>[2x]GQDLALSCGTSEASADQDKKKWEPDTKFLKTGNSIHATATYQDPSLLSTVPYMTARIFTAPATYEIPIKGDKRHLLRLYFYPSTYTGLNISNSYFTVEANDVTLLSNFSAAITCQALTQAYLVKEYSLAPTDKDVLSIKFTPSDKYRDAFAFINGIEVIQMPELFDTAALVGFTDQTMDAKTANLQSMFRLNVGGQDIPGSQDSGGLTRTWYNDAPYIFSAGLGVTLQASNNFRINYQNMP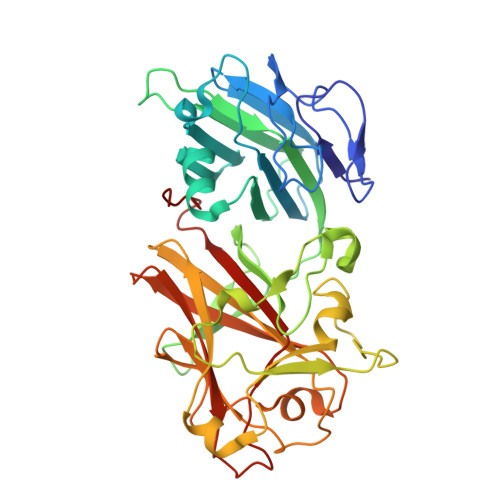VSIAPADIYKTARSQGPNGDINLKSNLTWMFQIDKNFTYILRLHFCEFQLSKINQKVFNIYINNRTAQADTTPADIIGWTGEKGIPMYKDYAIYVDANNGGEEITLQMTPSTFGQPEYYDSSLNGLEIFKMDTMKNLAGPNPEP>[2x]MFKHIIARTPARSLVDGLTSSHLGKPDYAKALEQHNAYIRALQTCDVDITLLPPDERFPDSVFVEDPVLCTSRCAIITRPGAESRRGETEIIEETVQRFYPGKVERIEAPGTVEAGDIMMVGDHFYIGESARTNAEGARQMIAILEKHGLSGSVVRLEKVLHLKTGLAYLEHNNLLAAGEFVSKPEFQDFNIIEI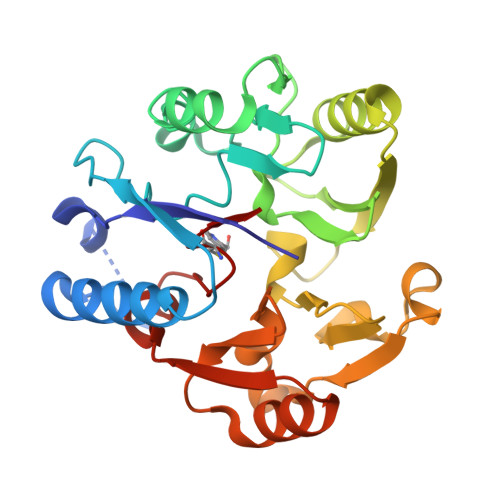PEEESYAANCIWVNERVIMPAGYPRTREKIARLGYRVIEVDTSEYRKIDGGVSCMSLRF> MECFVPLRCDLDGSNIEQLRQSHLSRKFIIFDEQLNLWLWFQGNSQENKRFVLQNMIILINEAQVTRTSTIDDYFTQVENNENLWRLKNDCCSKILFKSNVVMNNGYNNQIKFVFEYKSVDANFNNQDSLQDPQAKYTLDKYSSEEILPSFEPVYSWSSAATKSSKNTNNHLEKNNRATHRVSSKNSEVHEADVSRNPNTFTLKLQYPIFSLLNMRLRNISLKSEHCILSSLDFQTSKASEQLTKKFIYPQEHNSFLKLNFQEISYKLIDGTSQIELDPICPLKVPLTAFSYDSISATFKLVLLPKSTQPHRVKITLAYELELHPNLKLPVRTSWETEVTLKRSMPISSTSSQYSSNNNNTNHSASFNGAANNVNSGGLANLRLGGVSSSRFSLGAASTTSLVNSKLSNVKFKFINSNIKVIKGEKFTMRLQIINSSSSPLDLVVYYNNTINP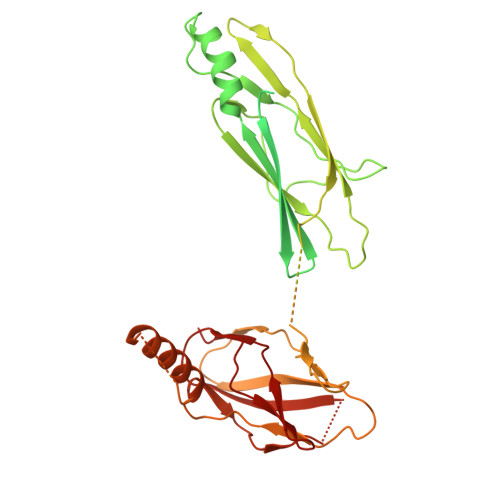IPSANNVRNSNGINNCGMNNGTIPNSPLTLENQYQLHNKYRKIAEGIILLSNDYKIPVVPPRETYFADLRFIGIMSGYYGTLSGLKVLDLNTNELIEVGNGASVLIQ4-{[6-(cyclohexylmethyl)pyridine-2-carbonyl]amino}-3-[(4-methoxyphenyl)amino]benzoic acid | C27 H29 N3 O4 | 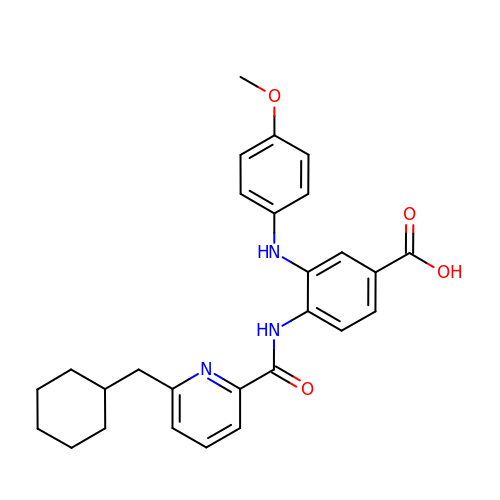HKIXXPHCIIDZPF-UHFFFAOYSA-N> MGVMNMREVVIASAARTAVGSFGGAFKSV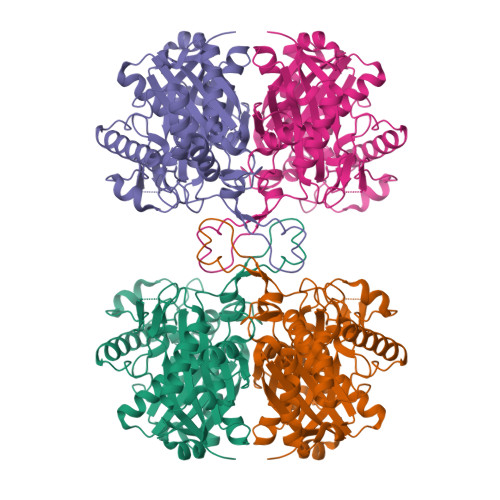SAVELGVTAAKEAIKRANITPDMIDESLLGGVLTAGLGQNIARQIALGAGIPVEKPAMTINIVCGSGLRSVSMASQLIALGDADIMLVGGAENMSMSPYLVPSARYGARMGDAAFVDSMIKDGLSDIFNNYHMGITAENIAEQWNITREEQDELALASQNKAEKAQAEGKFDEEIVPVVIKGRKGDTVVDKDEYIKPGTTMEKLAKLRPAFKKDGTVTAGNASGINDGAAMLVVMAKEKAEELGIEPLATIVSYGTAGVDPKIMGYGPVPATKKALEAANMTIEDIDLVEANEAFAAQSVAVIRDLNIDMNKVNVNGGAIAIGHPIGCSGARILTTLLYEMKRRDAKTGLATLCIGGGMGTTLIVKR>[2x]MAST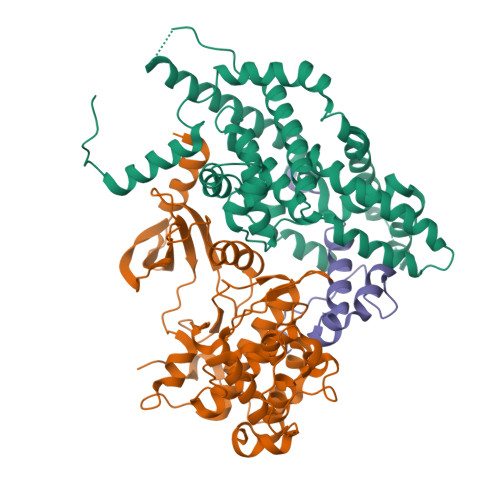IASEDARYRQSSQYELWSFSPSQLASMREKTNAAARARITERLLSMPNPSNTASAPTSSANTPDPDGVSTPTLPEFLTPAEELLLVTFYTAELLRAGDHADMSDEIKATAATFFKRFYITNSIMTYPPQEMLLVALFFGCKAEGAFPSISDFAKTFGRERPEEILAGEFLLCQGIRFALDVKHPFRALRGAIMELSTLPDVEPARLVAAEQRAREILRFSPLITDAYFHFTPSQIMLAALSLADRGLAERLIQDTFHYVAPQPSSGTDTPATSGVETPSGASASISLHKRTASPSSGSLEDKAAVIGSHVRDKVLGTIEACRDMLSKELPERREHWNNKTVYKAQIQPIRKKLNKCRDPDRWNLVELQRIRREQASRKGFDSDDEGEGRTKGGSLEDDAAVFGVPKKKKQLEDPFGPPLAG;>[2x]MAASPLIAPPTDALQQSRPGSTSSPFKRQPQQPSQPPSSTAPSSSNANDTPQLGSRPPNITIANVTSAPFSSRPAITPDPVEQMNEAEKRKYIKGKKLGEGTYANVYLGHSRDDPNFKVAIKKIKVQAQYKDGMAPDAVRELKYLRELRGHPNIIGLISVFSSKDQNLNLVLEYLPLGDLEMLIRDVERVRYGAADIKAWMGMLTRAVWWCHENFILHRDIKPNNLLIAADGEVKLADFGLARSFADPGRRMTANVITRWYRPPELLFGARHYGGAVDIWSVGMVFAELIIRSPFLPGNTEMEQITLICKHIGTPTEENWPGVSKLPEWWDPMEEPIPVWGKDAYMARFGAVGSEGVDLLWRTLQLDPKKRITAREMLEHRWWRTDPKPTRKEDLPKKSGGEDKMGADLKRRPGMVEDENGPRGSKVARKLDFGQLK;>[2x]GPYDPFGGMEFVPSRYRVREELNHPSLDKYRIDQQHITGGYSFLDYISRAMFEAFAGLAVFIEDEKEAG> MIPHSWICEKHILWLKDYKNSSNWKLFKECWKQGQPAVVSGVHKKMNISLWKAESISLDFGDHQADLLNCKDSIISNANVKEFWDGFEEVSKRQKNKSGETVVLKLKDWPSGEDFKTMMPARYEDLLKSLPLPEYCNPEGKFNLASHLPGFFVRPDLGPRLCSAYGVVAAKDHDIGTTNLHIEVDDVVNILVYVGIAKG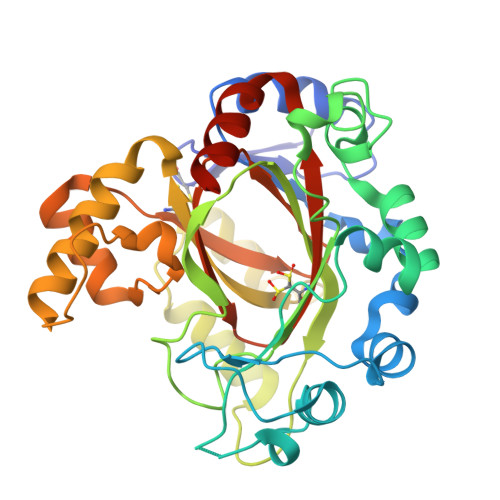NGILSKAGILKKFEEEDLDDILRKRLKDSSEIPGALWHIYAGKDVDKIREFLQKISKEQGLEVLPEHDPIRDQSWYVNKKLRQRLLEEYGVRTCTLIQFLGDAIVLPAGALHQVQNFHSCIQVTEDFVSPEHLVESFHLTQELRLLAENLYFQ CRISPR-associated transposons (CAST) are programmable mobile genetic elements that insert large DNA cargos using an RNA-guided mechanism. CAST elements contain multiple conserved proteins: a CRISPR effector (Cas12k or Cascade), a AAA+ regulator (TnsC), a transposase (TnsA–TnsB) and a target-site-associated factor (TniQ). These components are thought to cooperatively integrate DNA via formation of a multisubunit transposition integration complex (transpososome). Here we reconstituted the approximately 1 MDa type V-K CAST transpososome from Scytonema hofmannii (ShCAST) and determined its structure using single-particle cryo-electon microscopy.

TnsC has dedicated interaction interfaces with TniQ and TnsB. Full-length TnsB has a 52-residue-long flexible linker (residues 518–569), that connects the STC to the C-terminal ‘hook’ (TnsBhook, residues 570–584). TnsBhook serves as the point of contact with the TnsC filament body and is critically important for CAST transposition. In particular, the new interactions with the DNA backbone, involving R182 and K119 are supported by cryo-EM density. Furthermore, because these interactions are not observed in the TniQ–TnsC structure, this is not solely owing to the binding of TniQ, but must be related to R-loop formation, consistent with other reports.

>MTEAQAIAKQLGGVKPDDEWLQAEIARLKGKSIVPLQQVKTLHDWLDGKRKARKSCRVVGESRTGKTVACDAYRYRHKPQQEAGRPPTVPVVYIRPHQKCGPKDLFKKITEYLKYRVTKGTVSDFRDRTIEVLKGCGVEMLIIDEADRLKPETFADVRDIAEDLGIAVVLVGTDRLDAVIKRDEQVLERFRAHLRFGKLSGEDFKNTVEMWEQMVLKLPVSSNLKSKEMLRILTSATEGYIGRLDEILREAAIRSLSRGLKKIDKAVLQEVAKEYK[11x];>MIEAPDVKPWLFLIKPYEGESLSHFLGRFRRANHLSASGLGTLAGIGAIVARWERFHFNPRPSQQELEAIASVVEVDAQRLAQMLPPAGVGMQHEPIRLCGACYAESPCHRIEWQYKSVWKCDRHQLKILAKCPNCQAPFKMPALWEDGCCHRCRMPFAEMAKLQKV[2x];>[9x]IEVWDYEQLREEYGF> GSAKDPMQGFILHTQKVKDEDLIVYILSSKMLIKAYRFYGLRHSSILSGYKIDFALEENPSFLPRLKDVLHLGFLWIMQRDKMLIWQEFIRLLYRHLKDV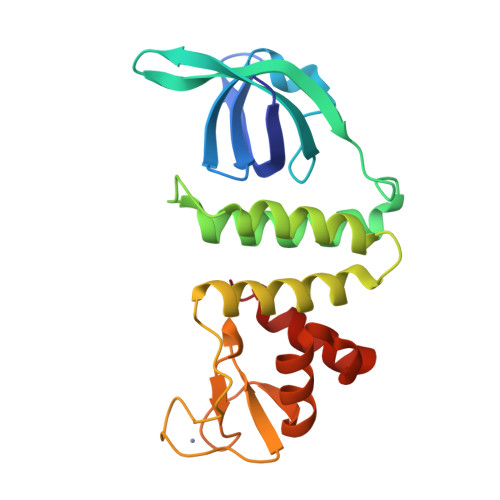EELDSFYFDLLDECVKRFEKQNPKRVIVDAYLKILEFEGRLHKDFFCFACDEKIQNSITLLRAFLPSHSQCALGFEFEEKKLKQFYSSKNCAIFDDEEIENLYHLIKEGL> GSHMDNQC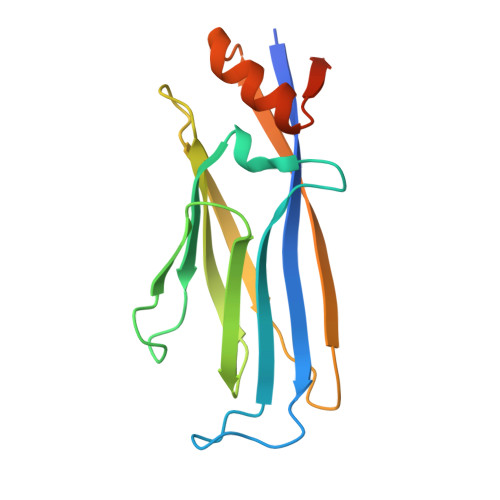TVQVRLELGHRAQLRKKPTTEGFTHDWMVFVRGPEQCDIQHFVEKVVFWLHDSFPKPRRVCKEPPYKVEESGYAGFIMPIEVHFKNKEEPRKVCFTYDLFLNLEGKVNHLRCEKLTFNNPTTEFRYKLLRAGGVMVMPEGAHHHHHH> MTTREYEEAFLPRRLKRIKVFNTPPPSELPAFFHKRLDNAHSNPRSILKLYRQYMRKDDYPAYDWLVRCFCHLGNVFGFNSFWATKDKQVIQALPSFKFLVYDLIERKHLIEARQVPRLLYAFACLEYRSWHLLPTLLEHVEANLEKWRTPTLANMALTLALLGVGDDAPDHNQFGPPD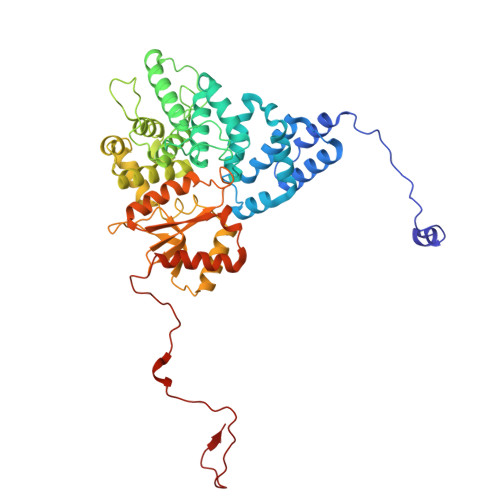LLSRDYTGLVSKLALEVHRRLLALQSASSSGPRKSPLHDSLGCMPFDYAGLAFALTLQGSYDLCLPSDETAKSTLALFLQRACEPLSLEQLENSGWVQFFLYQTLYCVDVEKPKREVEVKKAVPFAFQKHLHLSWLDKILINAQPQGNELLQLDVDAALKRLHITDALINCSAGRQWDEQHCWFAGHLVRSRNLALEYDYLLPLGPGRPKVSGWLACKRRMLKAFGLNVATIHQSFWSLLNLEQKDVQLTRLLAQFPPVLEAVKDEKKAYEEDRHLRFQRHARQKFETWPPEKLEI4-bromanylbenzenesulfonic acid | C6 H5 Br O3 S | 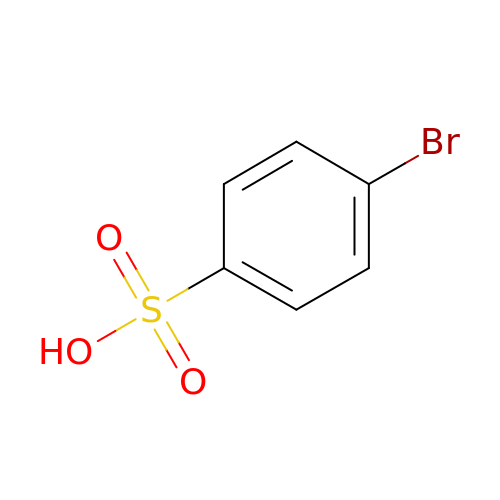PXACTUVBBMDKRW-UHFFFAOYSA-N> GLEAVRKRPGMYIGSTSGEGLHHLVWEIVDNSIDEALAGFAKSIQVIIEPDDSITVIDDGRGIPVGIQAKTGRPAVETVFTVLHAGGKFGGGGYKVSGGLHGVGSSVVNALSTSLDVRVYKDGKVYYQE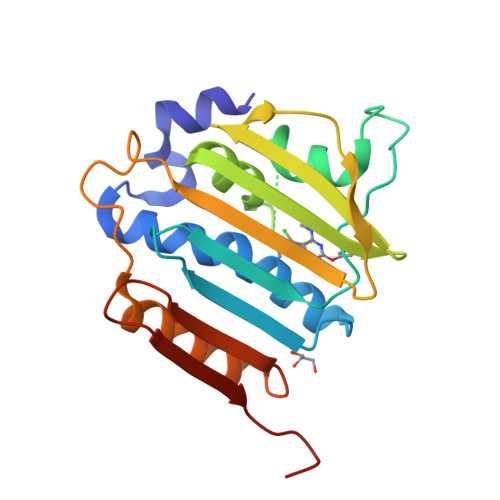YRRGAVVDDLKVIEETDRHGTTVHFIPDPEIFTETTVYDFDKLATRVRELAFLNRGLHISIEDRREGQEDKKEYHYEGLEHHHHHH> MSYASRTLGPMQTSSDRHEYPAHWEADVVLRDGGTARVRPITVDDAERLVSFYEQVSDESKYYRFFAPYPRLCAKDVHRFTHHDFVDRVGLAATIGGEFIATVRYDRIGAGGTPATAPADEAEVAFLVQDAHQGRGVASALLEHIAAVARERGIRRFAAEVLPANNKMIKVFMDAGYTQKRSFEDGVVRLEFDL;> DVLNVSGHRLGTAEIESALVAHPKIAEAAVVGIPHAIKGQ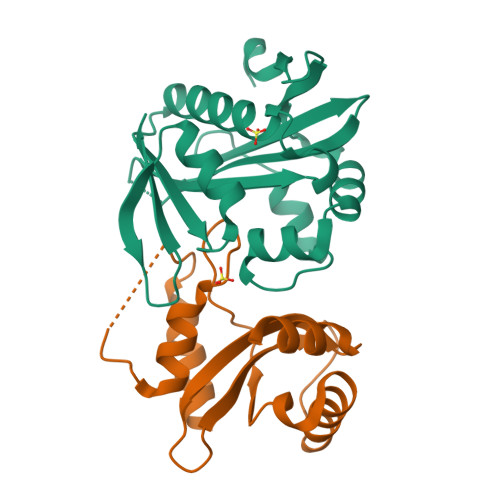AIYAYVTLNCGEEPSPELYAEVRNWVRKEIGPLATPDVLHWTDSLPKTRSGKIMRRILRKIAAGDTSNLGDTSTLADPGVVEKLLEEKQAIAMPS> MISLNGYGRFGLQYVEDRGVGLEDTIISSRLRINIVGTTETDQGVTFGAKLRMQWDDGDAFAGTAGNAAQFWTSYNGVTVSVGNVDTAFDSVALTWDSEMGYEASSFGDAQSSFFAYNWKYDASGALDNYNGIAVTYSISGVNLYLSYVDPDQTVDSSLVTEEFGIAADWSNDMISLAAAYTTDAGGIV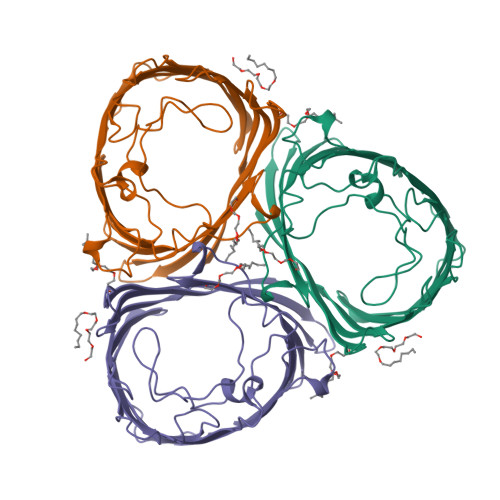DNDIAFVGAAYKFNDAGTVGLNWYDNGLSTAGDQVTLYGNYAFGATTVRAYVSDIDRAGADTAYGIGADYQFAEGVKVSGSVQSGFANETVADVGVRFDF>SVDLTVPWDDIEALLKNNF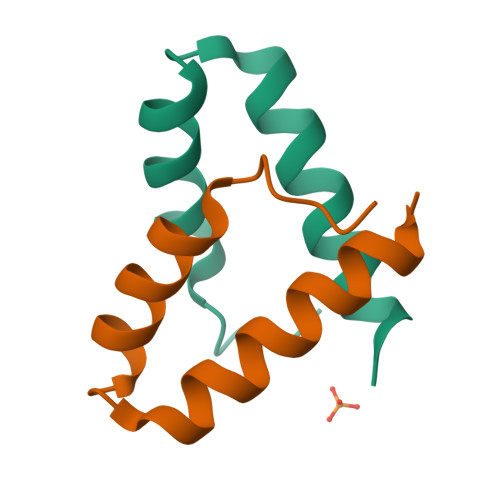ENDQAAVRQVMERLQKGWSLAK[2x]> MASNQELVQIATNFLLNAPPCEFMEVVSDVRALLPSESLLNASAGSTFREYNTSQMVSVQTSKGSALITKEGEISNNEYLDPKNKQVITYDHIKQEVTGERSASGEIEQDIEQYRAAFDEEATKYCNEYYPNGVSAVYGTKVSEGIKITVCISTCIYKPNAFYSGRWRSVWTCTFKPGSGNVTSNGKVQVNVHYFEDGNVQLNT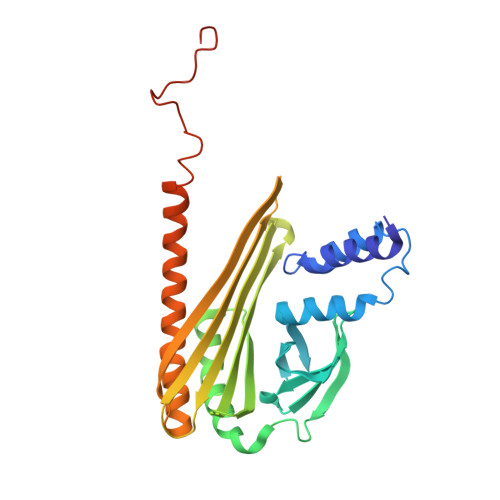VTQKQTTSPSADAQSTAVNAFKAIGKAELNLHTALDNNYSTMGDTTFKALRRALPINRTKINWQKVKNFKIANELNK>[2x]AEGTRGRSSTARCSLFGSDFVNTFDGSMYSFAGYCSYLLAGGCQKRSFSIIGDFQNGKRVSLSVYLGEFFDIHLFVNGTVTQGDQRVSMPYASKGLYLETEAGYYKLSGEAYGFVARIDGSGN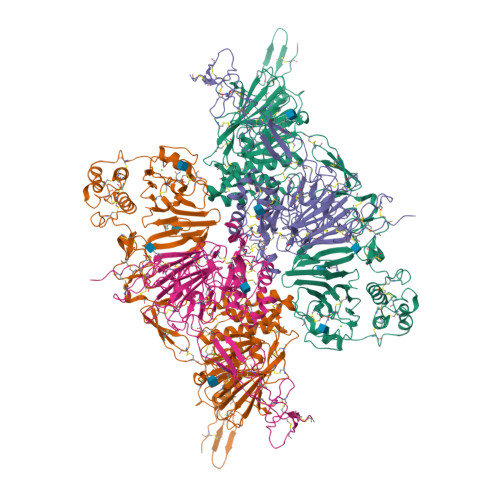FQVLLSDRYFNKTCGLCGNFNIFAEDDFMTQEGTLTSDPYDFANSWALSSGEQWCERASPPSSSCNISSGEMQKGLWEQCQLLKSTSVFARCHPLVDPEPFVALCEKTLCECAGGLECACPALLEYARTCAQEGMVLYGWTDHSACSPVCPAGMEYRQCVSPCARTCQSLHINEMCQERCVDGCSCPEGQLLDEGLCVESTECPCVHSGKRYPPGTSLSRDCNTCICRNSQWICSNEECPGECLVTGQSHFKSFDNRYFTFSGICQYLLARDCQDHSFSIVIETVQCADDRDAVCTRSVTVRLPGLHNSLVKLKHGAGVAMDGQDVQLPLLKGDLRIQHTVTASVRLSYGEDLQMDWDGRGRLLVKLSPVYAGKTCGLCGNYNGNQGDDFLTPSGLAEPRVEDFGNAWKLHGDCQDLQKQHSDPCALNPRMTRFSEEACAVLTSPTFEACHRAVSPLPYLRNCRYDVCSCSDGRECLCGALASYAAACAGRGVRVAWREPGRCELNCPKGQVYLQCGTPCNLTCRSLSYPDEECNEACLEGCFCPPGLYMDERGDCVPKAQCPCYYDGEIFQPEDIFSDHHTMCYCEDGFMHCTMSGVPGSLLPDAVLSSPLSHRSKR;>SLSCRPPMVKLVCPADNLRAEGLECTKTCQNYDLECMSMGCVSGCLCPPGMVRHENRCVALERCPCFHQGKEYAPGETVKIGCNTCVCQDRKWNCTDHVCDATCSTIGMAHYLTFDGLKYLFPGECQYVLVQDYCGSNPGTFRILVGNKGCSHPSVKCKKRVTILVEGGEIELFDGEVNVKRPMKDETHFEVVESGRYIILLLGKALSVVWDRHLSISVVLKQTYQEKVCGLCGNFDGIQNNDLTSSNLQVEEDPVDFGNSWKVSSQCADTRKVPLDSSPATCHNNIMKQTMVDSSCRILTSDVFQDCNKLVDPEPYLDVCIYDTCSCESIGDCACFCDTIAAYAHVCAQHGKVVTWRTATLCPQSCEERNLRENGYECEWRYNSCAPACQVTCQHPEPLACPVQCVEGCHAHCPPGKILDELLQTCVDPEDCPVCEVAGRRFASGKKVTLNPSDPEHCQICHCDVVNLTCEACQEPGGLVVPPHHHHHH[2x]> QWMEGNGPAAVHYQPASPPRDACVYSSCYSEENVWKLCEYIKNHDQYPLEECYAVFISNERKMIPIWKQQARPGDGPVIWDYHVVLLHVSSGGQSFIYDLDTVLPFPCLFDTYVEDAIKSDDDIHPQFRRKFRVICADSYLKNFASDRSHM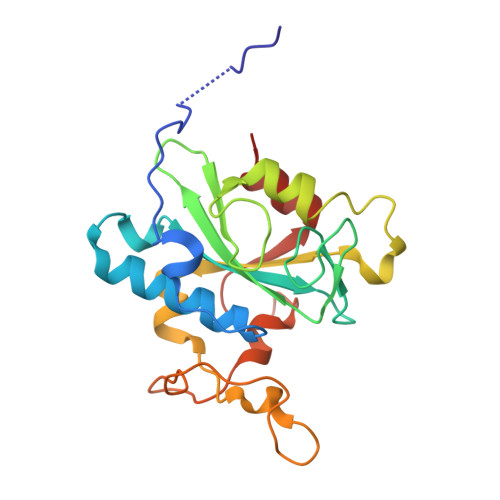KDSSGNWREPPPPYPCIETGDSKMNLNDFISMDPKVGWGAVYTLSEFTHRFGS> GMDVVDPDIFNRDPRDHYDLLQRLGGGTYGEVFKARDKVSGDLVALKMVKMEPDDDVSTLQKEILILKTCR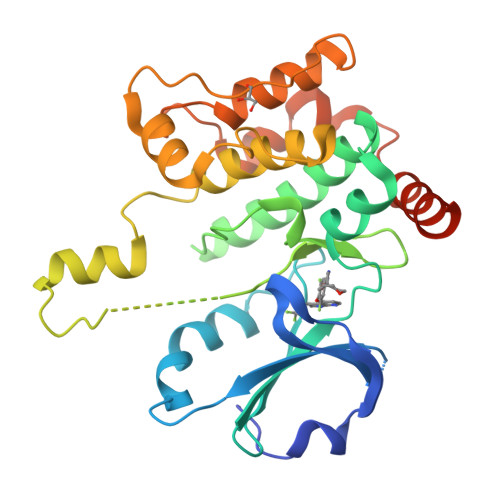HANIVAYHGSYLWLQKLWICMEFCGAGSLQDIYQVTGSLSELQISYVCREVLQGLAYLHSQKKIHRDIKGANILINDAGEVRLADFGISAQIGAELARRLEFIGTPYWMAPEVAAVALKGGYNELCDIWSLGITAIELAELQPPLFDVHPLRVLFLMTKSGYQPPRLKEKGKWSAAFHNFIKVTLTKSPKKRPSATKMLSHQLVSQPGLNRGLILDLLDKLKNPGKGPSIGDIEDEE>[6x]MVPDRREQSKAKERLLEREEALAKHMSEREKRPPPKIDPPPSPKAPEPSKRVLKEKQAPLFVDTAVEGTLPPLSLLDPAEVKQKSYSPESLEAMSRLLEIKLKEFGVEVSVDSVHPGPVITRFEIQPAAGVKVSRISNLAKDLARSLAVISVRVVEVIPGKTTVGIEIPNEDRQMVRFSEVLSSPEYDEHKSTVPLALGHDIGGRPIITDLAKMPHLLVAGTTGSGKSVGVNAMLLSILFKSTPSEARLIMIDPKMLELSIYEGIPHLLCPVVTDMKEAANALRWSVAEMERRYRLMAAMGVRNLAGFNRKVKDAEEAGTPLTDPLFRRESPDDEPPQLSTLPTIVVVVDEFADMMMIVGKKVEELIARIAQKARAAGIHLILATQRPSVDVITGLIKANIPTRIAFQVSSKIDSRTILDQGGAEQLLGHGDMLYLPPGTGLPIRVHGAFVSDDEVHRVVEAWKLRGAPDYIEDILAGVDEGGKLHHHHHH

Among them, the bacterial protein FtsK is unusual in that it translocates on double-stranded DNA and is also the fastest known translocase. FtsK is an essential part of the bacterial cell division machinery, recruiting downstream factors through its N-terminal transmembrane domain. Its C-terminal cytoplasmic domain, which follows an often very long linker domain, can be subdivided into three modules: α, β, and γ, with β adopting the RecA-fold that contains the ATPase activity. Upon recognition by the γ module of one direction-determining sequence in the genome, named KOPS (FtsK-orienting polar sequences), α and β oligomerize as a homo-hexameric ring around double-stranded DNA (dsDNA) (forming FtsKαβ-dsDNA). To this end, we solved by electron cryo-microscopy (cryo-EM) structures of FtsKαβ from Pseudomonas aeruginosa bound to dsDNA.

The FtsKαβ-dsDNA-ATPγS sample was much more heterogeneous, the particles less symmetrical, and the DNA generally much better defined after three-dimensional (3D) refinement. Overall, three main particle classes could be distinguished, II.A, III.B, and III.E, each accounting for 4.9, 4.3, and 5.2%, respectively, of total particles selected after 2D classification and pruning for highest quality. States II.A and III.B were reconstructed to 3.99 and 4.34 Å resolution and are in very similar conformations. Both structures are moderately asymmetric, mostly due to a movement of the β-subdomains in subunits A and B, turned away from the α-ring. Other subunits are again very similar to the previous crystallographic structure. The main difference between these two states lies in the length of the resolved dsDNA, which is 5 bp shorter in II.A on the side closest to the β-subdomain at the pore entry. From the maps we determined that in these structures ADP occupies all nucleotide-binding pockets, which suggests that they represent stalled states, with II.A having reached the end of the short 45-bp DNA after translocation.>[2x]GTGVQENRTKTTDSPAKLKCPKDWHSHQDKCFHVSQTSITWKG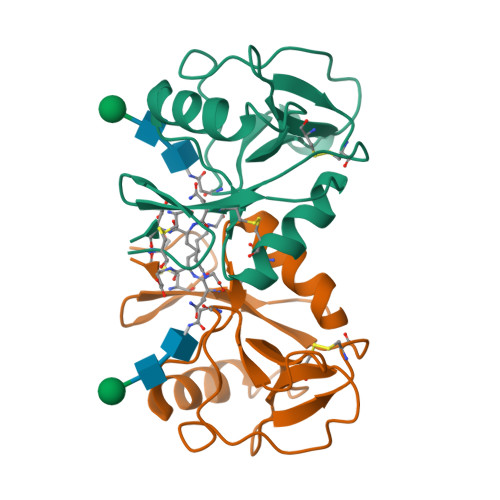SLADCGGKGATLLLVQDQEELRFLRNLTKRISSSFWIGLSYTLSDEKWKWINGSTLNSDALNITGDTEKDSCASVSQDKVLSESCDSDNIWICQKELKRESTCNDS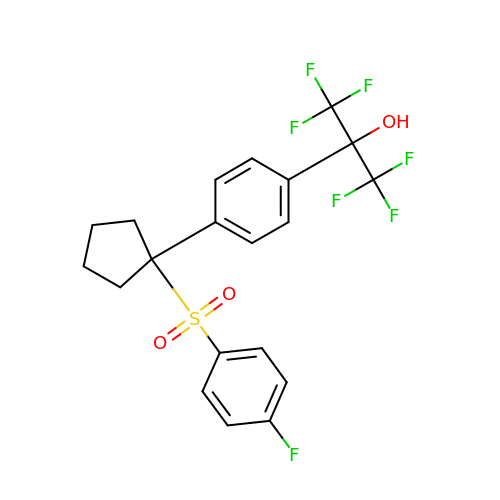1,1,1,3,3,3-hexafluoro-2-(4-{1-[(4-fluorophenyl)sulfonyl]cyclopentyl}phenyl)propan-2-ol | C20 H17 F7 O3 S | BANKSZZTXXTYRE-UHFFFAOYSA-N[[(2~{R},3~{S},4~{R},5~{R})-5-[2,4-bis(oxidanylidene)pyrimidin-1-yl]-3,4-bis(oxidanyl)oxolan-2-yl]methoxy-oxidanyl-phosphoryl] [(2~{R},3~{R},4~{R},5~{R},6~{R})-3-(hex-5-ynoylamino)-6-(hydroxymethyl)-4,5-bis(oxidanyl)oxan-2-yl] 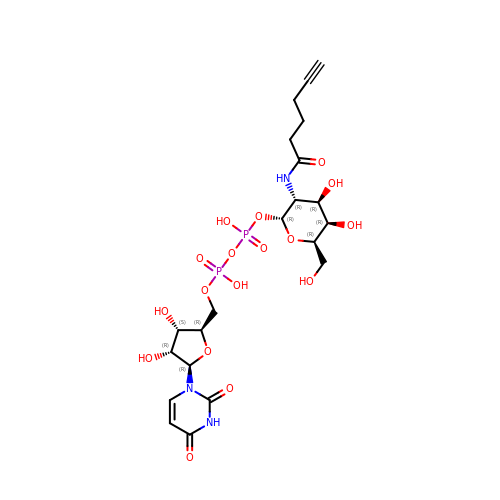hydrogen phosphate | C21 H31 N3 O17 P2 | SPUYDPWWABYYLH-SSBRDYMUSA-N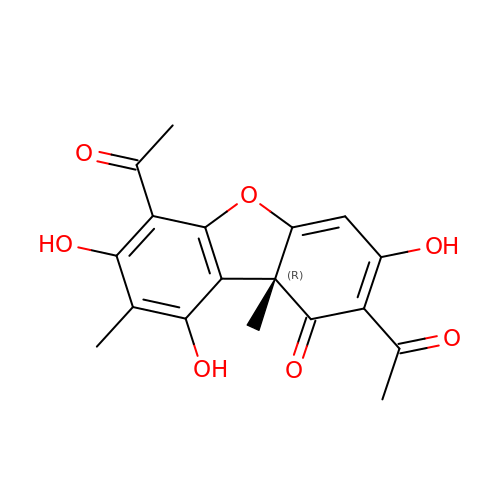(9bR)-2,6-diethanoyl-8,9b-dimethyl-3,7,9-tris(oxidanyl)dibenzofuran-1-one | C18 H16 O7 | WEYVVCKOOFYHRW-SFHVURJKSA-N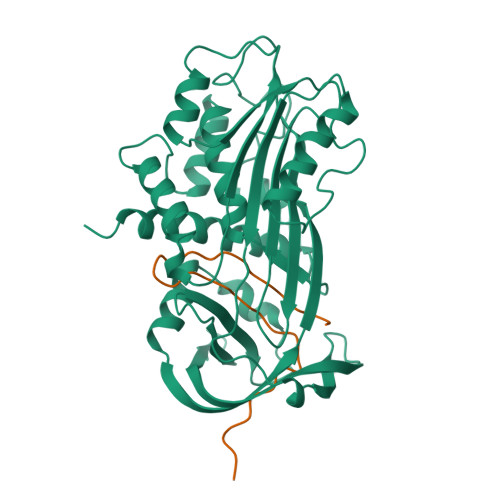> VHHPPSYVAHLASDFGVRVFQQVAQASKDRNVVFSPYGVASVLAMLQLTTGGETQQQIQAAMGFKIDDKGMAPALRHLYKELMGPWNKDEISTTDAIFVQRDLKLVQGFMPHFFRLFRSTVKQVDFSEVERARFIINDWVKTHTKGMISNLLGKGAVDQLTRLVLVNALYFNGQWKTPFPDSSTHRRLFHKSDGSTVSVPMMAQTNKFNYTEFTTPDGHYYDILELPYHGDTLSMFIAAPYEKEVPLSALTNILSAQLISHWKGNMTRLPRLLVLPKFSLETEVDLRKPLENLGMTDMFRQFQADFTSLSDQEPLHVAQALQKVKIEVNESGTVPSSSTAVIVSAR;> MAPEEIIMDRPFLFVVRHNPTGTVLFMGQVMEP> LPTSNPAQELEARQLGRTTRDDL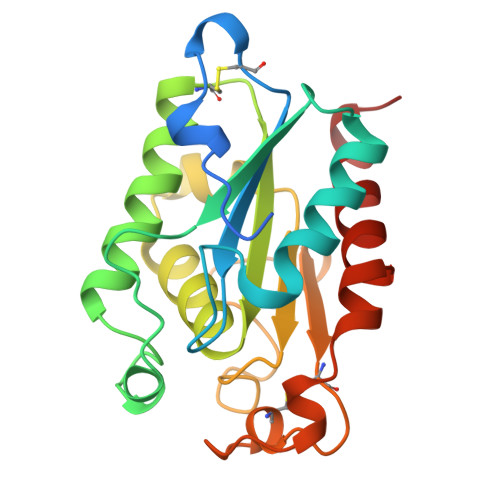INGNSASCRDVIFIYARGSTETGNLGTLGPSIASNLESAFGKDGVWIQGVGGAYRATLGDWALPRGTSSAAIREMLGLFQQANTKCPDATLIAGGYSQGAALAAASIEDLDSAIRDKIAGTVLFGYTKNLQNRGRIPNYPADRTKVFCNTGDLVCTGSLIVAAPHLAYGPDARGPAPEFLIEKVRAVRGSA>NIGSQWRDDEVHFNRTLDSILVPRVVGSRGHQQVREYLVQSLNGLGFQTEVDEFKQRVPVFGELTFANVVGTINPQAQNFLALAAHYDSKYFPNDPGFVGATDSAVPAAILLNTAKTLGAYLQKEFRNRSDVGLMLIFFDGEEAFKEWTDADSVYGSKHLAAKLASKRSGSQAQLAPRNIDRIEVLVLLDLIGARNPKFSSFYENTDGLHSSLVQIEKSLRTAGQLEGNNNMFLSRVSGGLVDDDHRPFLDENVPVLHLVATPFP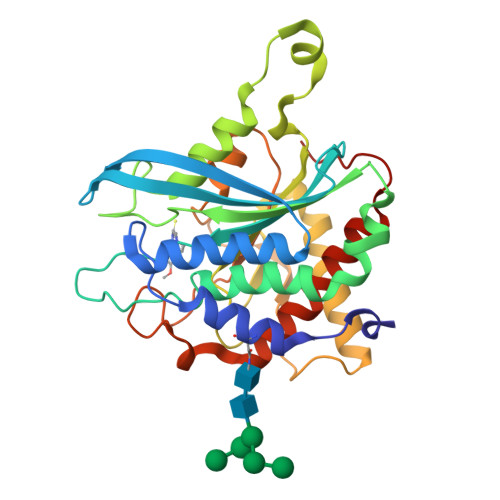DVWHTPRDNAANLHWPSIRNFNRVFRNFVYQYLKRHTSPVNLRFYRT[2x]> IVGGYTCAANSIPYQVSLNSGSHFCGGSLINSQWVVSAAHCYKSRIQVRLGEHNIDVLEGNEQFINAAKIITHPNFNGNTLDNDIMLIKLSSPAT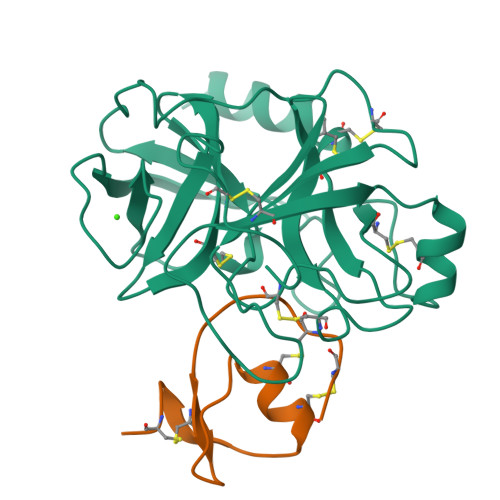LDSRVATVSLPRSCAAAGTECLISGWGNTKSSGSSYPSLLQCLKAPVLSDSSCKSSYPGQITGNMICVGFLEGGKDSCQGDSGGPVVCNGQLQGIVSWGYGCAQKNKPGVYTKVCNYVNWIQQTIAAN;> KKVCACPKILKPVCGSDGRTYANSCIARCNGVSIKSEGSCPTGILN>MSLKIRDAYTIVTCPGRNFVTLKIVTESGTHGIGDATLNGREMAVAAYLDEHVVPALIGRDAGRIEDTWQYLYRGAYWRRGPVTMTAIAAVDMALWDIKAKAAGMPLYQLLGGKSRERVMTYAHCTGQTIEDCLGEVARHVELGYRAVRVQSGVPGIETTYGVAKTPGERYEPADSSLPAEHVWSTEKYLNHAPKLFAAVRERFGDDLHVLHDVHHRLTPIEAARLGKAVEPYHLFWLEDCVPAENQESLRLIREHTTTPLAIGEVFNSIHDCRELIQNQWIDYIRMPLTHGGGITAMRRVADLASLYHVRTGFHGPTDLSPVCLGAAIHFDTWVPN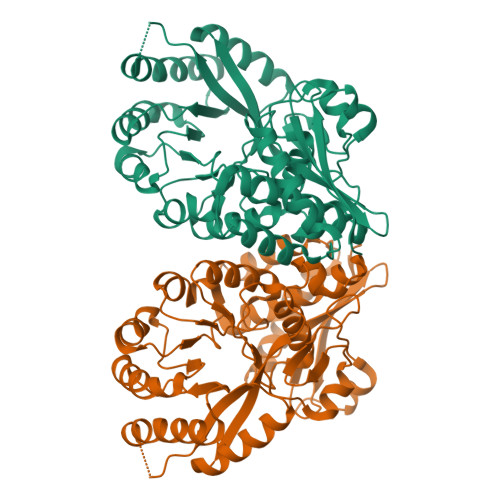FGIQEHMPHTDETDAVFPHDYRFEDGHFLAGESPGHGVDIDEELAAKYPYERASLPVNRLEDGTLWHWEGHHHHHH[4x]> GSFTDEDDWSKPLPPSERLEQELFSGGNTGINFEKYDDIPVEATGNNCPPHIESFSDVEMGEIIMGNIELTRYTRPTPVQKHAIPIIKEKRDLMACAQTGCGKTAAFLLPILSQIYSDGPGEALRAMKENGRYG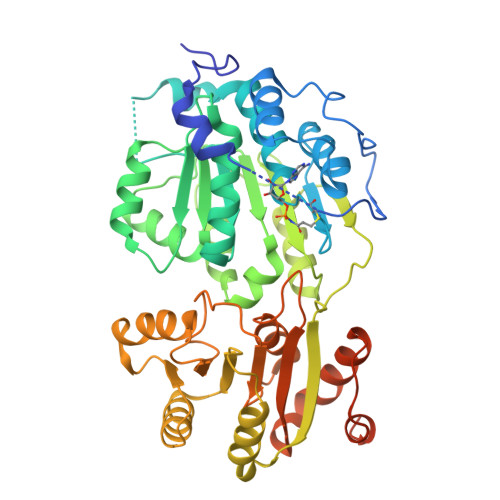RRKQYPISLVLAPTRELAVQIYEEARKFSYRSRVRPCVVYGGADIGQQIRDLERGCHLLVATPGRLVDMMERGKIGLDFCKYLVLDEADRMLDMGFEPQIRRIVEQDTMPPKGVRHTMMFSATFPKEIQMLARDFLDEYIFLAVGRVGSTSENITQKVVWVEESDKRSFLLDLLNATGKDSLTLVFVETKKGADSLEDFLYHEGYACTSIHGDRSQRDREEALHQFRSGKSPILVATAVAARGLDISNVKHVINFDLPSDIEEYVHRIGRTGRVGNLGLATSFFNERNINITKDLLDLLVEAKQEVPSWLENMAYEHHYKGSSRGRSKSSRFSGGFGARDYRQSSG> GSNGAIPFPVGSLPGTAPCGFVVSDALEPDNPIIYVNTVFEIVTGYRAEEVIGRNCRFLQCRGPFTKRRHPMVDSTIVAKMRQCLE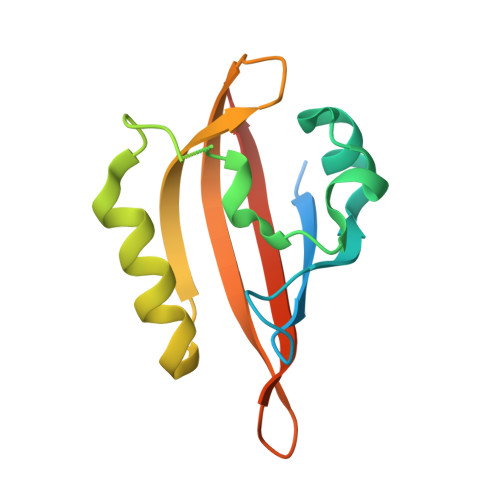NGIEFQGELLNFRKDGSPLMNKLRLVPIREEDEITHFIGVLLFTDAKIDLGP>[2x]MGTTYTIFGAGPAGLYTAWRLVTGGKAVAGDTIQLYEWGDYAFDGPGSGTRLPAGRIVTHFCNDDPKQSYIEAGGMRFIEWDGTKSQGHQLVTLTIQALGLSGKVIDFNTTDNPLLFLREEHIYQNDLATHPAPYNTPGNNEQPAATLFSNISALITGDAPVSTRTQQCAFYGSGRLPSTFNSFVYPPGSIAGNIGYWNVFYDQAGNEGYEYAADAGGYTSNVINWNAANAAVYNGEFAPGGAFKTVNGGYSQVFVQLYQQTLAAAQEAGVAFTLTQRTRLHSVWLEDDVVNYRLASAENPFKGGAVQTTQNAFLAMPPASLD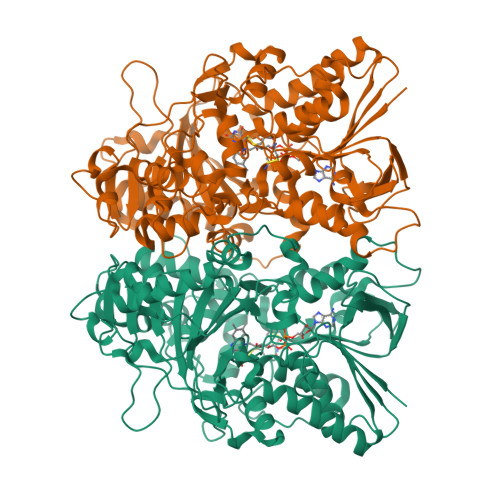LVAEATRYADMPEGTLDILNAEGVQLYMDGVIRQPSMRVMLFFDRPWWTDADVPYPPDLTSDGAPNTFGPTITDLPLRQVYYFGNNSDGTANPVYGVLASYDDMQYVQFWQELEIDVGERRKVPIDQDYQVLFGPRKATDTMIRMVLLELAKVHWGDPNAAHQIPWPVEAIFNDFSLNPFGAGYHAWAAHYDICDVMQRIRQPTGLVPGATAANLFIIGEAYSNDQAWVEGAFCTAESVLVDYYGMTTIADTTNYPLICACPLEHHHHHH>RASQQIPWGIKAIYNNDTLTSTTGGSGINIAVLDTGVNTSHPDLVNNVEQCKDFTGATTPINNSCTDRNGHGTHVAGTALADGGSDQAGIYGVAPDADLWAYKVLLDSGSGYSDDIAAAIRHAADQATATGTKTIISMSLGSSANNSLISSAVNYAYSKGVLIVAAAGNSGYSQGTIGYPGALPNAIAVAALENVQQNGTYRVADYSSRGYISTAGDYVIQEGDIEISAPGSSVYSTWYNGGYNTISGTSMATPHVSGLAAKIWA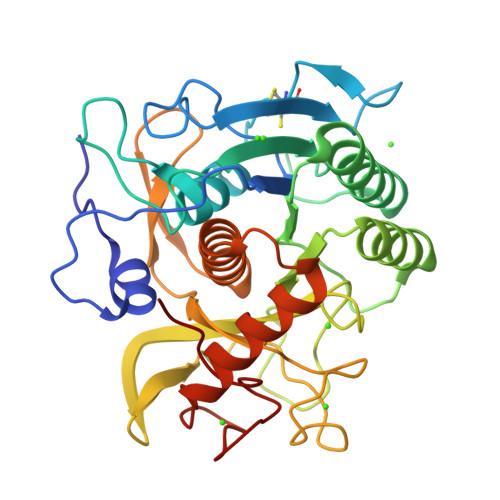ENPSLSNTQLRSNLQERAKSVDIKGGYGAAIGDDYASGFGFARVQ[2x]> HHHH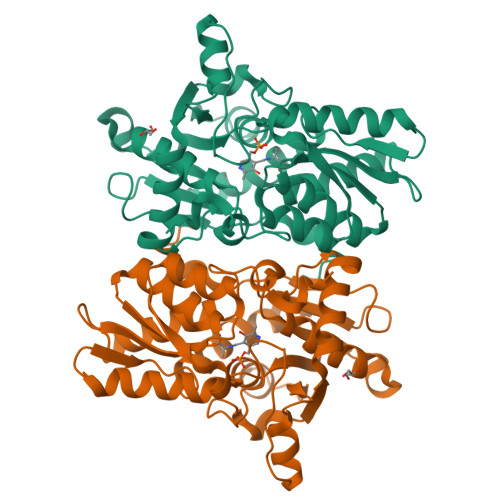HHMAIYADNSYSIGNTPLVRLKHFGHNGNVVVKIEGRNPSYSVKCRIGANMVWQAEKDGTLTKGKEIVDATSGNTGIALAYVAAARGYKITLTMPETMSLERKRLLCGLGVNLVLTEGAKGMKGAIAKAEEIVASDPSRYVMLKQFENPANPQIHRETTGPEIWKDTDGKVDVVVAGVGTGGSITGISRAIKLDFGKQITSVAVEPVESPVISQTLAGEEVKPGPHKIQGIGAGFIPKNLDLSIIDRVETVDSDTALATARRLMAEEGILAGISSGAAVAAADRLAKLPEFADKLIVVILPSASERYLSTALFEGIEG(2Z,4E)-5-[(1S)-1-hydroxy-2,6,6-trimethyl-4-oxocyclohex-2-en-1-yl]-3-methylpenta-2,4-dienoic 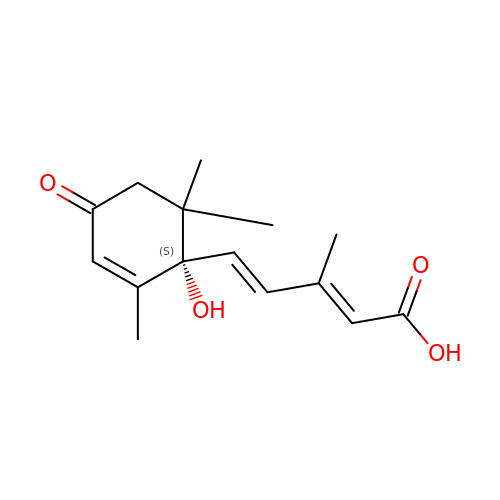acid | C15 H20 O4 | JLIDBLDQVAYHNE-YKALOCIXSA-N>[2x]SFRDNLKVYIESPESYKNVIYYDDDVVLVRDMFPKSKMHLLLMTRDPHLTHVHPLEIMMKHRSLVEKLVSYVQGDLSGLIFDEARNCLSQQLTNEALCNYIKVGFHAGPSMNNLHLHIMTLDHVSPSLKNSAHYISFTSPFFVKIDTPTSNLPTRGTLTSLFQEDLKCWRCGETFGRHFTKLKAHLQEEYDDWLDKSVSM

We reported previously that the DNA repair enzyme aprataxin has a DNA 3′ de-capping activity, converting DNAppG to DNA3′p and GMP. Aprataxin catalyzes the conversion of A5′pp5′DNA to AMP and pDNA via a covalent enzyme-(histidinyl)–AMP intermediate. Aprataxin consists of two modules: a proximal HIT domain and a C-terminal zinc-finger. The HIT domain is organized around a central 6-strand antiparallel β-sheet that, along with flanking loops and helices, forms the NMP-binding pocket.

In order to gain insights to how aprataxin recognizes the DNA 3′ cap, we grew crystals of the catalytic domain of S. pombe aprataxin that had been preincubated with GMP, the product of the DNAppG de-capping reaction, and determined the structure at 1.5 Å resolution. The crystals contained two aprataxin protomers in the asymmetric unit. The refined model included guanosine in the active site of the A protomer and GMP in the active site of the B protomer, in identical positions and anti nucleoside conformations. The phosphate is flanked by the catalytic His138, His147, and His149 side chains. The planar purine ring of the guanine nucleobase is sandwiched by van der Waals contacts to Leu38 and Met64. The striking feature of the guanine-bound aprataxin is an extensive hydrogen bonding network to the O6, N1, N2 edge of the nucleobase. The Tyr41 hydroxyl engages in direct bifurcated hydrogen bonds to the guanine N1 and N2 atoms and in a water-bridged contact to the guanine O6. The guanine N2 atom is contacted by the Arg62 main-chain carbonyl and the Asn50 side chain (which in turn, makes bridging hydrogen bonds to Tyr41-OH and Arg62-O). Asp63 is a bidentate acceptor of hydrogen bonds from the 2′-OH and 3′-OH groups. Lys67 makes a direct hydrogen bond to the 2′-OH and a water-mediated contact to the 3′-OH.>[2x]SNALTPPPDSKISTTDKSLDKLSAPLDMLKQMNESTMEQTKLDELRKKMSLQAEILNKAKADNDMFFRLLIELMSLKLQGELFKEQLSKISKESGYDSAQSALIQATNSEGQSPLQYALQKQDFSTAKYFLDNGAKAGPIEKAVFEIALDSKAAKEFGFPPLPPEKEKLHPVKNFGLVLGIKTTSVDGTPSQFGHIAPTYQLMTDSVSHFAKSHPGNKNFQEIANAFQF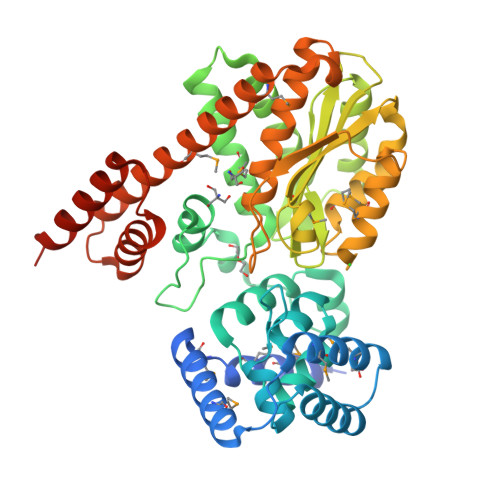SNEASAFKFSTPQRNPEAGNDLARRIQGGELTTIPVSCKGHAMGLSYVPDGPGSKSGYLVYTNRGLGAKSSEHGTHIFRIEDSSKITPEFINNMTSGHSNGASHDEIMSQIKAAAGNKEPIHHIKQKGQKNDNCTIANSKSNIEGILLCQKAREVGGFDKLTESDMDSVKKEYKEFTKHMRVEKVNELAKALKENPQDPDLNNLTKEYLKQHPNADPKLKQTLETALKQASESSMTLSQPGKTI> MASHSRKFLDVRSEEELLSCIKKETEAGKLPPNVAAGMEELYQNYRNAVIESGNPKADEIVLSNMTVALDRILLDVEDPFVFSSHHKAIREPFDYYIFGQNYIRP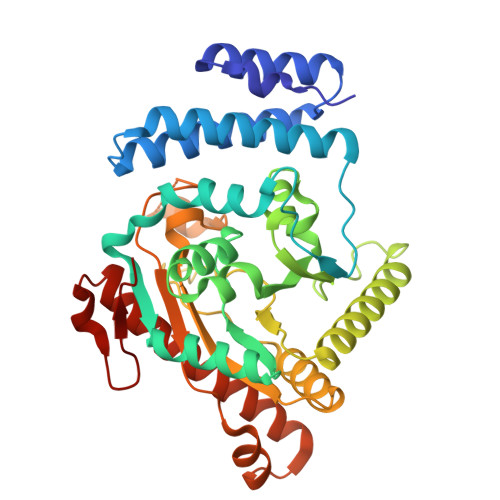LIDFGNSFVGNLSLFKDIEEKLQQGHNVVLISNHQTEADPAIISLLLEKTNPYIAENTIFVAGDRVLADPLCKPFSIGRNLICVYSKKHMFDIPELTETKRKANTRSLKEMALLLRGGSQLIWIAPSGGRDRPDPSTGEWYPAPFDASSVDNMRRLIQHSDVPGHLFPLALLCHDIMPPPSQVEIEIGEKRVIAFNGAGLSVAPEISFEEIAATHKNPEEVREAYSKALFDSVAMQYNVLKTAISGKQGLGASTADVSLSQPW> GPHMLELTKEQLYQQAMEEAAWHHMPHPSDSERIRQYLPRNPCPTPPYHHQMPPPHSDTVEFYQRLSTETLFFIFYYLEGTKA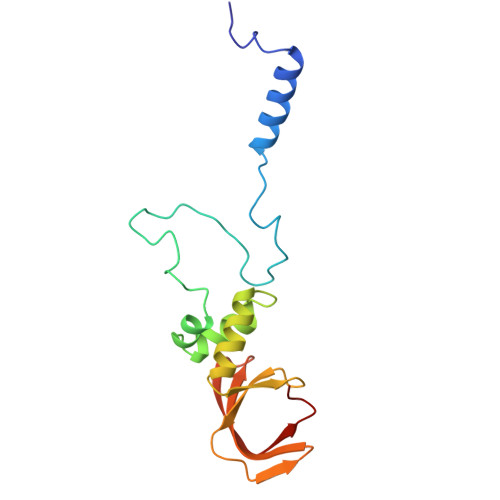QYLAAKALKKQSWRFHTKYMMWFQRHEEPKTITDEFEQGTYIYFDYEKWGQRKKEGFTFEYRYLE> MPALPEDGGSGAFPPGHFKEPKRLYCKNGGFFLRIHPDGRVDGVREKSDPHIKLQLQAEERGVVSIKGVLANRYLAMKEDGRLLASKIVTDECFFFERLESNNYNTYRSRKYTSWYVALKRTGQYKLGPKTGPGQKAILFLPMSAKS

Canonical FGFs including FGF2 act as a paracrine and/or an autocrine by forming ternary complexes with FGF receptors (FGFRs) and heparan sulfate proteoglycans (HSPGs) on the cell surface. The FGFR-FGF-HSPG complex induces the dimerization of FGFR, resulting in a series of intracellular signaling cascades including the activation of MAPK/ERK pathway, PI3K/AKT pathway, and PLCγ pathway, etc. Through these signaling pathways, FGF2 regulates diverse cellular responses and has beneficial effects on wound healing, wrinkle reduction, and protection against neomycin-induced hair cell loss. While the therapeutic potentials of FGF2 are widely recognized, a significant challenge hindering its broader application is inherent instability.

To improve the thermo-stability of FGF2, we designed two mutants harboring four-point mutations: FGF2-M1 (D28E/C78L/C96I/S137P) and FGF2-M2 (D28E/C78I/C96I/S137P) through bioinformatics, molecular thermodynamics, and molecular modeling. We successfully solved the high-resolution (1.40 Å and 1.48 Å, respectively) crystal structures of FGF2-M1 and the FGF2-M2/SOS complex. The crystallization of FGF2-M1 was successful in the absence of SOS. The RMSD value between the structures of the FGF2 mutants was 0.144 Å for all Cα atoms, indicating that the introduction of mutations did not affect the overall structure of FGF2. The D28E mutation is situated at the end of the N-terminal loop (residues 20–28 in the structure of FGF2-M1) independent from the β-trefoil fold of FGF2. The B´ value of the N-terminal loop was 2.82 Å2, suggesting that the region could be structurally disordered and easily exposed to protease. Structural analysis of the model structure showed that the side chain of D28E was at least 7.5 Å away from the surface of FGFR1c, indicating that the mutation at position 28 only confers resistance to fragmentation of FGF2 without affecting its interaction with FGFR1c. P137 is located at the end of the β11 strand and contacts with the side-chain indole ring of W123, positioned at the beginning of the β10 strand. It has been established that the electron-rich π face of the indole ring forms a CH-π interaction with the partially positively charged hydrogen atoms adjacent to the carbonyl and amide nitrogen of P137. Therefore, S137P seems to improve the thermo-stability of FGF2 by anchoring the beginning and end of the β10–β11 hairpin such as a knot.> HGHINDIVINGVWYQAYDPTTFPYESNPPIVVGWTAADLDNGFV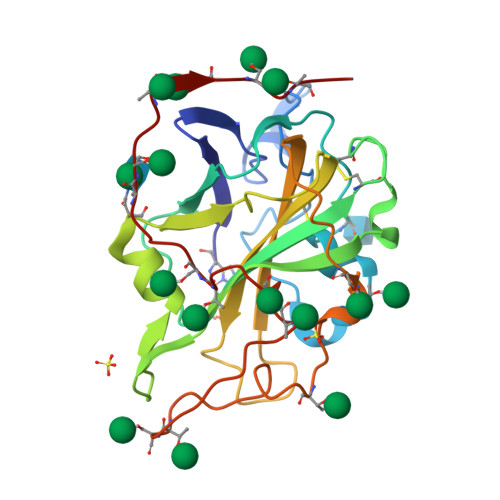SPDAYQNPDIICHKNATNAKGHASVKAGDTILFQWVPVPWPHPGPIVDYLANCNGDCETVDKTTLEFFKIDGVGLLSGGDPGTWASDVLISNNNTWVVKIPDNLAPGNYVLRHEIIALHSAGQANGAQNYPQCFNIAVSGSGSLQPSGVLGTDLYHATDPGVLINIYTSPLNYIIPGPTVVSGLPTSVAQGSSAATATASATVP Peptidyl-prolyl isomerases (PPIases) catalyze intrinsically slow and often rate-limiting isomerization of prolyl-peptide bonds in unfolded or partially folded proteins, thereby speeding up the folding process and preventing misfolding. An example of such a protein is SlyD (Sensitive to Lysis D), which consists of an FKBP type PPIase domain and a chaperone domain, called IF (insert-in-flap) domain, that has been shown to exhibit chaperone activity. Each of these domains contains one binding site for unfolded proteins or peptides. Often, FKBPs are linked to an additional chaperone domain that can increase their PPIase activity by up to 200-fold.

We measured the rate of prolyl isomerization in the presence of wild-type SlyD (SlyDWT) and a construct lacking the IF chaperone domain (SlyDΔIF). In contrast, the activity of SlyDΔIF on the peptide carrying the mutation M8A is increased. The crystal structure of SlyDΔIF complexed with the M8A substrate offers hints to an additional feature of the chaperone domain that could contribute to increased activity. In this structure, the PPIase domain architecture is well conserved (RMSD of Cα of the core FKBP domain of SlyDWT—residues 1–57 and 126–150—and SlyDΔIF is 0.80 Å), but the peptide M8A is bound in an inverse direction. We could model 14 residues of the substrate peptide that displays an opposite directionality compared with SlyDWT. However, this peptide binding mode is not possible in case of the peptide M8A in SlyDWT because the bulky side chain of the tryptophan in position 4 of the peptide would sterically clash with the β8-β9 hairpin of the chaperone domain. In our structures described here, we have observed the same substrate bound now in two different orientations in the absence and in the presence of the chaperone domain, implying that the chaperone domain binding provides directionality for substrate binding in the PPIase domain thereby leading to increased activity, by preventing unproductive binding. First, the chaperone domain can contribute to the directionality of the substrate binding in the PPIase domain, as is apparent from our crystal structures of a peptide substrate bound in a reverse direction in the absence of chaperon domain.

>[2x]MKVGQDKVVTIRYTLQVEGEVLDQGELSYLHGHRNLIPGLEEALEGREEGEAFQAHVPAEKAYGATGHPGIIPPHATLDFQVEVVKVREATPEELLHGHAHPSGHHHHHH;>TRYWNAKALPFAFGA[2x]(2S)-2-[[(2R)-2-[(2R,3R,4R,5S,6R)-3-acetamido-2-[[[(2R,3S,4R,5R)-5-[2,4-bis(oxidanylidene)pyrimidin-1-yl]-3,4-bis(oxidanyl)oxolan-2-yl]methoxy-oxidanyl-phosphoryl]oxy-oxidanyl-phosphoryl]oxy-6-(hydroxymethyl)-5-oxidanyl-oxan-4-yl]oxypropanoyl]amino]-3-oxidanyl-propanoic 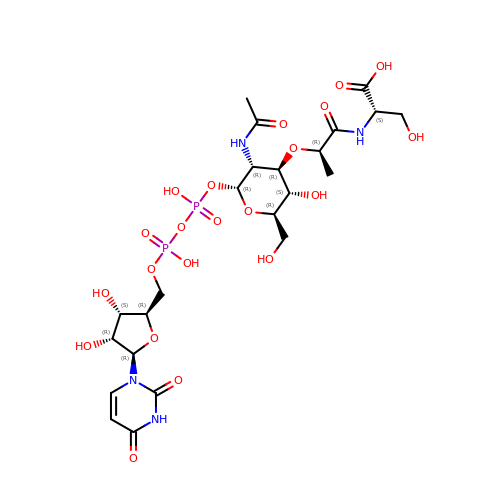acid | C23 H36 N4 O21 P2 | IACRIBHKJKCIBJ-KWWGHZHGSA-N>GPLGSPEFPGRPAFEGLVQRIRLIVPSTLRGGDGEAGPYSPSSLPSRCAFQFHGHDGSDESFPIEYVLRLMNDWAEVPCNPYLRIQNTGVSVLFQGFFHRPHNAPGGAITPERTNVILGSTETTGLSLGDLDTIKGRLGLDARPMMASMWISCFVRMPRVQLAFRFMGPEDAGRTRRILCRAA[6x];>[6x]GPGSQELCLHERQRYRGLFAALAQTPSEEIAIVRSLSVPLVKTTPVSLPFCLDQTVADNCLTLSGMGYYLGIGGCCPACNAGDGRFAATSREALILAFVQQINTIFEHRAFLASLVVLADRHNAPLQDLLAGILGQPELFFVHTILRGGGACDPRLLFYPDPTYGGHMLYVIFPGTSAHLHYLLIDRMLTACPGYRFVAHVWQSTFVLVVRRNAEKPTDAEIPTVSAADIYCKMRDISFDGGLMLEYQRLYATFDEFPPP

UL31 is a soluble nuclear phosphoprotein whereas UL34 is a type I membrane protein containing a single C-terminal transmembrane helix. Together, UL31 and UL34 form the heterodimeric nuclear egress complex (NEC) that is anchored in the INM and faces the nuclear interior. Composed of the viral proteins UL31 and UL34, NEC deforms the membrane around the capsid as the latter buds into the perinuclear space. In HSV-1 NEC, oligomerization into the hexagonal lattice is essential for budding.

Interestingly, the nuclear budding defect due to the DNUL34 mutation could be suppressed by an extragenic mutation in HSV-1 UL31, R229LUL31, which arose during serial passaging of the DNUL34 mutant HSV-1 virus on a UL34-complementing cell line through directed viral evolution [reviewed in [29,30]]. We refer to this mutation as SUPUL31. To obtain a high-resolution view of the hexagonal lattice formed by the NEC-SUPUL31 mutant, we crystallized the NEC185Δ50-SUPUL31 and the NEC185Δ50-DNUL34/SUPUL31 constructs, the mutant equivalents of the previously crystallized WT NEC185Δ50 construct (UL31: 51–306 and UL34: 15–185). Both mutants took the space group C21 with six crystallographically independent NEC heterodimers in the asymmetric unit, SUPAB, SUPCD, SUPEF, SUPGH, SUPIJ, and SUPKL (UL34 chains: A, C, E, G, I, and K; UL31 chains: B, D, F, H, J, and L). The NEC185Δ50-SUPUL31 structure was refined to 3.9-Å resolution. Nonetheless, the NEC185Δ50-SUPUL31 hexamers looked very similar to the WT NEC185Δ50 hexamers, with similar hexameric interfaces. The R229LUL31 mutation eliminated this salt bridge, and in all SUPUL31 heterodimers (except for SUPKL where it was unresolved), the D129UL31 side chain pointed away from L229UL31. The lack of the R229UL31-D129UL31 salt bridge in the NEC-SUPUL31 structure correlated with an ordered 129UL31-134UL31 loop. Importantly, some of the new contacts at the interhexameric interface were mediated by the 129UL31-134UL31 and 261UL31-268UL31 loops that were ordered in the NEC-SUPUL31 but not the WT NEC structures. Therefore, in the NEC-SUPUL31 mutant, there were new contacts at the interhexameric interface that could, in principle, stabilize the NEC lattice in the presence of lattice-destabilizing mutations.> GPISPIETVPVKLKPGMDGPKVKQWPLTEEKIKALVEICTEMEKEGKISKIGPENPYNTPVFAIKKKDSTKWRKLVDFRELNKRTQDFWEVQLGIPHPAGLKKKKSVTVLDVGDAYFSVPLDEDFRKYTAFTIPSINNETPGIRYQYNVLPQGWKGSPAIFQSSMTKILEPFKKQNPDIVIYQYMDDLYVGSDLEIGQHRTKIEELRQHLLRWGLTTPDKKHQK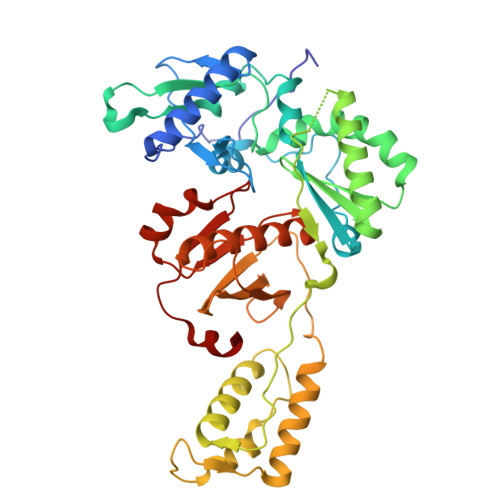EPPFLWMGYELHPDKWTVQPIVLPEKDSWTVNDIQKLVGKLNWASQIYPGIKVRQLSKLLRGTKALTEVIPLTEEAELELAENREILKEPVHGVYYDPSKDLIAEIQKQGQGQWTYQIYQEPFKNLKTGKYARMRGAHTNDVKQLTEAVQKITTESIVIWGKTPKFKLPIQKETWETWWTEYWQATWIPEWEFVNTPPLVKLWYQ>[6x]MPVSNAQLTQMFEHVLKLSRVDETQSVAVLKSHYSDPRTVNAAMEAAQRLKAKVYAVELPAFNHPTAMGNDMTAYCGDTALTGNLAAQRALEAADLVVDTMMLLHSPEQEQILKTGTRILLAVEPPEVLARMLPTEDDKRRVLAAETLLKQARSLHVRSKAGSDFHAPLG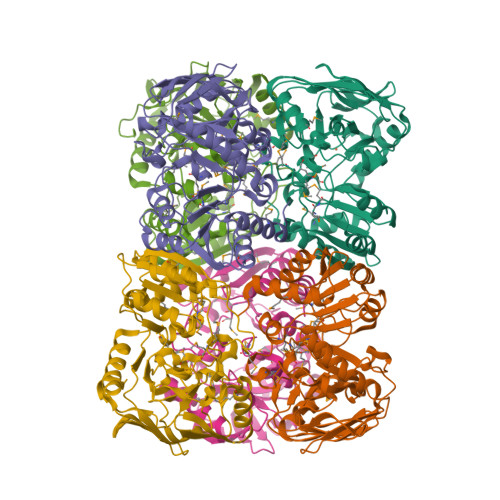QYPAVTEYGYADEPGRWDHWPSGFLFTWPNEDSAEGTLVLDVGDIILPFKNYCRERITLEIEKGFITGIHGGFEAEYLRDYMKYFNDPEVYGISHIGWGLQPRAQWTAMGLHDRNDGMCMDARAFYGNFLFSTGPNTEVGGKRKTPCHLDIPLRNCDIYLDDKAVVLAGDVVAPEESRARKLAAALEHHHHHH> MSGDENPASKPTPVQDVQGDGKWMSLHHRFVADSKDKEPEVVFIGDSLVQLMHQCEIWRELFSPLHALNFGIGGDSTQHVLWRLENGELEHIRPKIVVVWVGTNNHGHTAEQVTGGIKAIVQLVNERQPQARVVVLGLLPR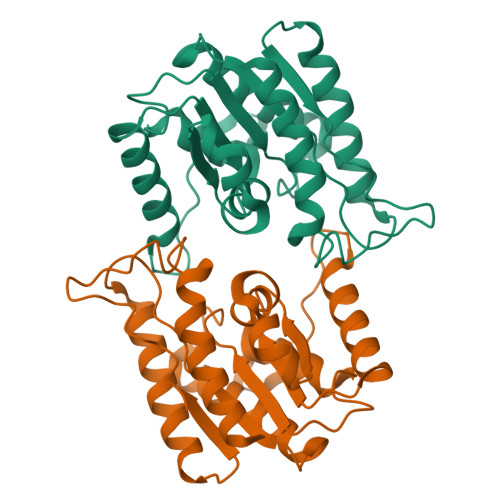GQHPNPLREKNRRVNELVRAALAGHPRAHFLDADPGFVHSDGTISHHDMYDYLHLSRLGYTPVCRALHSLLLRLLTQDQGQGGAPLPEPSP5-({[4-({4-[3-chloro-5-(trifluoromethyl)phenyl]piperazin-1-yl}sulfonyl)phenyl]carbamoyl}amino)-N-hydroxypentanamide 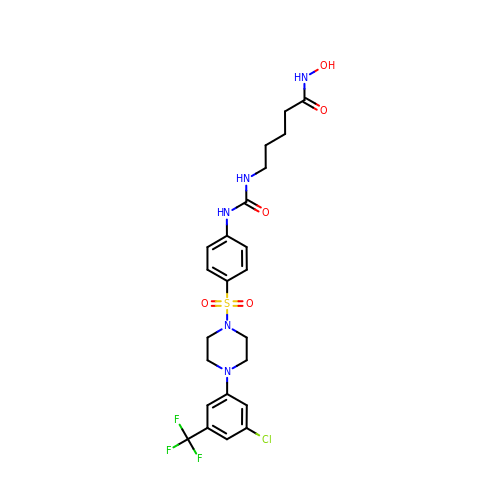| C23 H27 Cl F3 N5 O5 S | YNBLMVJKYWHKRJ-UHFFFAOYSA-N>VDISTLPRVKVDLVKPPFVHAHDQVAKTGPRVVEFTMTIEEKKLVIDREGTEIHAMTFNGSVPGPLMVVHENDYVELRLINPDTNTLLHNIDFHAATGALGGGALTQVNPGEETTLRFKATKPGVFVYHCAPEGMVPWHVTSGMNGAIMVLPRDGLKDEKGQPLTYDKIYYVGEQDFYVPKDEAGNYKKYETPGEAYEDAVKAMRTLTPTHIVFNGAVGALTGDHALTAAVGERVLVVHSQANRDTRPHLIGGHGDYVWATGKFRNPPDLDQETWLIPGGTAGAAFYTFRQPGVYAYVNHNLIEAFELGAAGHFK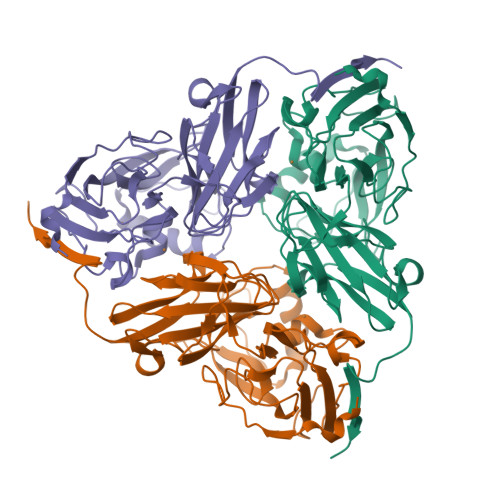VTGEWNDDLMTSVVKPASM[3x]The Vip3 (vegetative insecticidal protein 3) family proteins from Bacillus thuringiensis convey toxicity to species within the Lepidoptera, and have wide potential applications in commercial agriculture. The Vip3 proteins have molecular masses of ~90 kDa, and are secreted as soluble proteins that form tetramers in solution. They can be proteolytically processed by trypsin or insect gut extracts to yield products of ~65 kDa and ~21 kDa that remain closely associated in solution. Vip3 proteins are proposed to exert their insecticidal activity through pore formation, though to date there is no mechanistic description of how this occurs on the membrane.

To investigate the structure and activity of proteolytically cleaved Vip3Bc1, we performed a trypsin digest to yield two primary digestion fragments of ~68 kDa and ~21 kDa respectively, which we term activated Vip3Bc1 (Vip3Bc1act). Mass spectrometry analysis indicates that these fragments are formed primarily by digestion at K205. We obtained a 3D reconstruction of the digested complex by single particle cryo-EM analysis to a global resolution of 4.8 Å (0.143 FSC threshold). The structures reveal that Vip3Bc1 to VipBc1act transition requires extensive conformational rearrangements, but consistent with previous biochemical analyses, retains its tetrameric state8 while opening an approximately 5 Å pore. We were not able to directly observe density for an extended alpha-helical bundle in our single particle cryoEM reconstruction of Vip3Bc1act, however we were able to use deposited Vip3Aa16 coordinates to generate a model for Vip3Bc1act EM density due to high sequence identity (59.9%). We observed that Vip3Bc1act associated with the membrane in an elongated ‘open umbrella’ conformation, ~15–18 nm on its longest dimension to the membrane, with a stalk interacting with the membrane and the bulk of the protein density distal to the membrane. B Scaled comparison between segmented density for a single particle in the tomogram, with 5 nm scale bar (i) compared to Vip3Bc1act model (ii) with an overlay showing the stalk density fits the 4-helix bundle well, and the density which is distal to the membrane is consistent with single particle Vip3Bc1act model. The helical stalk modelled in Vip3Bc1act does not account for all of the stalk density observed in the sub-volume. Following cleavage, inter-subunit interactions at the conical tip of the complex dissociate, allowing for helices α1–α3 to rotate and move down through the gap between the ‘propeller’ regions of adjacent monomers, and form the extended helical bundle at the base of the complex, as visualised via cryoET and consistent with the reports for Vip3Aa1616.

>MVQKWMQRMIIVDNNKLNVRALPSFIDYFNGIYGFATGIKDIMGMIFKTDTGGSNLTLDEILKNQNLLNDISGKLDGINGDLGDLIAQGNLNSELAKELLKISNEQNQMLNHVNAQLNAINSTLNIYLPKITSMLNEVMKQNHVLSLQIEFLSKQLQEISDKLDIINLNVLINSTLTEITPAYQRIKYVNEKFDELTSTVEKNPKSYQDNVTKEVIENLNELTELAKSVTKNDMDSFEFYLQTFHDVMTGNNLFGRSALKTASELITKENVTTRGSEIGKVYNFLIVLTSLQAKAFLTLTACRKLLGLTDIDYTQIMNHHIDGQKREFRINILPTLSNNFSNPSYSKNRGSDIDDPIVVLEAAPGYALIGFEILNDPLPILKGYQARLKPNYQVDRESMSETIYGDIHKLFCPKQLEQKYYIKDIEFPEGYVITKIVFEKRLNQLGYEVTANFYDPSTGSIDLNKVKVESWKEKSCEEDSCEDEYSIIKAETDGIYMPLGVVSETFLTPIYGFGLTVDEKNQKITLTGKSYLRESLLETDLLNNETYLIASPDGYISSIVENWNITSDNTGSWRANNNNAFVDKADTIKGSSSLYTHKDGEFSQFIGNKLKPKTNYVIQYVIKGRPAIYLKNNKDTLFEDTKNNFSDFQTVTKKFNSGVNPSEIYFLFKNQSEYEAWGNNFIILEIKSLEFLPQMLKPEDWIPSGNVQMKDGGRLEILGDGYFKQFIKLENDSTYHLRLSVKGTGRVSIIDESKYLLFVNVKDEDLTRVIKNTSSKGECFIALEGTYVENSSTIFSNVSIVKE[4x]>[2x]QEQVAPPKDPAAALEDHKTRTDNRYEPSLDNLAQQDVAAPGAPEGVSALSDAQYNEANKIYFERCAGCHGVLRKGATGKALTPDLTRDLGFDYLQSFITYGSPAGMPNWGTSGELSAEQVDLMANYLLLDPAAPPEFGMKEMRESWKVHVAPEDRPTQQENDWDLENLFS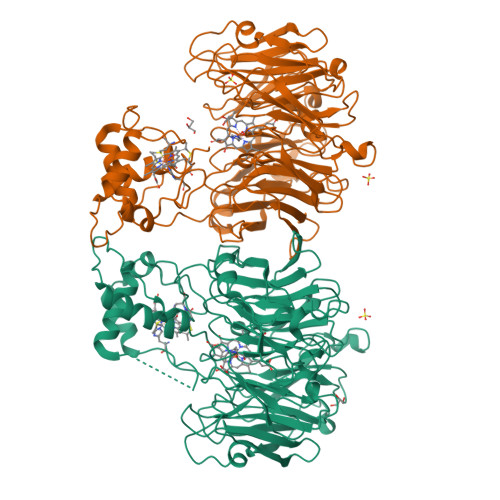VTLRDAGQIALIDGATYEIKSVLDTGYAVHISRLSASGRYLFVIGRDGKVNMIDLWMKEPTTVAEIKIGSEARSIETSKMEGWEDKYAIAGAYWPPQYVIMDGETLEPKKIQSTRGMTYDEQEYHPEPRVAAILASHYRPEFIVNVKETGKILLVDYTDLDNLKTTEISAERFLHDGGLDGSHRYFITAANARNKLVVIDTKEGKLVAIEDTGGQTPHPGRGANFVHPTFGPVWATSHMGDDSVALIGTDPEGHPDNAWKILDSFPALGGGSLFIKTHPNSQYLYVDATLNPEAEISGSVAVFDIKAMTGDGSDPEFKTLPIAEWAGITEGQPRVVQGEFNKDGTEVWFSVWNGKDQESALVVVDDKTLELKHVIKDERLVTPTGKFNVYNTMTDTY Escherichia coli YtfE is a di-iron protein of the widespread Repair of Iron Centers proteins (RIC) family that has the capacity to donate iron, which is a crucial component of the biogenesis of the ubiquitous family of iron-sulfur proteins. Bacterial RICs are composed by an N-terminal ScdA-like domain and a C-terminal domain that folds as a four-helix bundle where a histidine/carboxylate di-iron type center is inserted. In E. coli YtfE, the best studied RIC protein, the center is coordinated by H84, H129, H160, H204, and two μ-carboxylate bridges formed by E133 and E208. We show that YtfE establishes protein-protein interactions with the scaffold IscU, where the transient cluster is formed, and the cysteine desulfurase IscS.

Crystals of E. coli YtfE could only be obtained when the proteins contained the mutation to alanine of the two vicinal cysteines C30 and C31 (designated YtfEM), a result that agrees with previous reports. The structure of E. coli YtfEM contains two channels. One channel is mainly hydrophobic (which will not be addressed in this study), and a second hydrophilic channel that connects the metal center to the solvent. The di-iron center is located ca. 10 Å below the channel entrance, which is approximately circular in shape with a diameter of ∼2.3 Å. The channel is formed mainly by hydrophilic residues, namely H160 and H129 (that are also Fe ligands), K132, E159, E125, and E162. The three negatively charged glutamates are located at the channel entrance and solvent exposed suggesting a possible iron exit. In YtfEM, hydrogen bonds occur between residues D5 and R17, E49, and R86. Analysis of the electrostatic potential on the molecular surface of E. coli YtfEM shows that domain A is mainly positively charged and domain B is mainly negatively charged. In addition, the cavity where the di-iron center is inserted is positively charged, and the negative charge at the surface in this region is mainly due to residues E125, E159, and E162. Besides these coordinating ligands, an oxo-bridge between the iron atoms is also present in YtfE.

>AYRDQPLGELALSIPRASALFRKYDMDYAAGGKQTLARAAARKELDVEVIEAELAKLAEQPIEKDWRSAPLAEIIDHIIVRYHDRHREQLPELILQATKVERVHADKPSVPKGLTKYLTMLHEELSSHMMKEEQILFPMIKQGMGSQAMGPISVMESEHDEAGELLEVIKHTTNNVTPPPEACTTWKAMYNGINELIDDLMDHISLENNVLFPRALAGE[2x]Citrate synthase (CS, EC 2.3.3.1), an enzyme involved in the TCA cycle, catalyzes the condensation of oxaloacetate and acetyl-coenzyme-A (CoA) to form citrate and CoA. Thermoacidophilic archaeon Sulfolobus tokodaii strain 7, which grows optimally at 75°C and pH 3, has two genes encoding two distinct isozymes of hypothetic CS. One of them encoded by an open reading frame (ORF) ST1805 is termed ST1805-CS, and the other, encoded by the ORF ST0587, is termed ST0587-CS. We confirmed these two isozymes to function in high temperatures as CS and determined the crystal structures of them at resolutions of 2.0 Å and 2.7 Å, respectively.

ST1805-CS is related closely to CS from the same genus Sulfolobus solfataricus (SS-CS), and they share 68% amino acid sequence identity. ST1805-CS crystallized in a monoclinic crystal belonging to P21 that diffracted X-rays up to 2.0 Å resolution. In this crystal, the asymmetric unit contains two monomers having nearly identical overall structures. The final model is comprised of 376 amino acid residues per subunit (two residues in the N-terminus are disordered), 341 water molecules, a glycerol molecule, and a sulfate ion. In the dimeric structure, each subunit is subdivided into a large domain with 11 α-helices (C-G, I-M, and S helices, residues 3–216 and 325–378) and a small domain with five α-helices (N-R helices, residues 217–324). The dimeric structure is further strengthened by an extended C-terminal loop, which involves a β-strand interacting with the first β-strand (residues 13–17) in the N-terminus of the other subunit. In the hinge region in subunit A of ST1805-CS, a glycerol molecule interacts with two glycine residues (Gly220, Gly 221) and interacts with His219 with a sulfate ion. His184, His259, Arg268, Arg339, and Arg359′, which are important residues for substrate binding, are exposed to the inner surface of the open cleft. In ST1805-CS, three arginine-glutamate pairs Arg370-Glu56′, Glu368-Arg30′, and Arg356-Glu10′ are formed, of which the new β-strand made across both termini from each subunit lies between the former two pairs and the latter one. In ST1805-CS, an ion pair network was comprised of three residues; Asp109 in GI loop and Asp202 in LM loop were salt-bridged with Lys215′ in M′N′ loop of neighboring subunit.

>MSVEVSRGLENVIIKTTGLTYIDGINGILRYRGYDINDLVNYASYEELIHLMLYGELPNRQQLNQIKGIINESFEVPEQVISTIFSMPRNCDAIGMMETAFGILASIYDPKWNRATNKELAVQIIAKTATITANIYRAKEGLKPKIPEPSESYAESFLAATFGKKPTQEEIKAMDASLILYTDHEVPASTTAALVASSTLSDMYSCIVAALAALKGPLHGGAAEEAFKQFVEIGSVENADKWFEEKIIKGKSRLMGFGHRVYKTYDPRAKIFKTLAKSFAEKNENVKKYYEIAERIEKLGVDTFGSKHIYPNTDFYSGIVFYALGFPIYMFTSLFALSRVLGWLAHIIEYVEEQHRLIRPRALYIGPEKREFKPIELR[2x]>[2x]MFHSSAMVNSHRKPMFNIHRGFYCLTAILPQICICSQFSVPSSYHFTEDPGAFPVATNGERFPWQELRLPSVVIPLHYDLFVHPNLTSLDFVASEKIEVLVSNATQFIILHSKDLEITNATLQSEEDSRYMKPGKELKVLSYPAHEQIALLVPEKLTPHLKYYVAMDFQAKLGDGFEGFYKSTYRTLGGETRILAVTDFEPTQARMAFPCFDEPLFKANFSIKIRRESRHIALSNMPKVKTIELEGGLLEDHFETTVKMSTYLVAYIVCDFHSLSGFTSSGVKVSIYASPD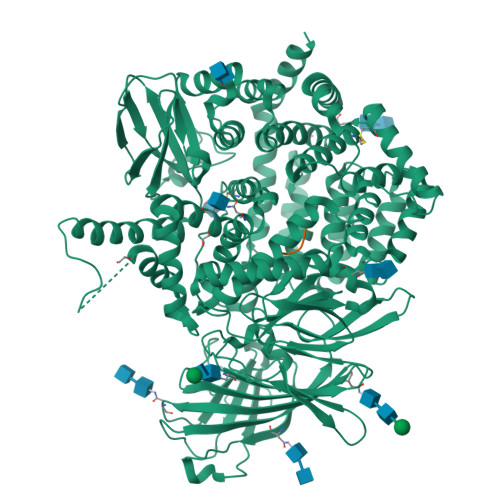KRNQTHYALQASLKLLDFYEKYFDIYYPLSKLDLIAIPDFAPGAMENWGLITYRETSLLFDPKTSSASDKLWVTRVIAHELAHQWFGNLVTMEWWNDIWLKEGFAKYMELIAVNATYPELQFDDYFLNVCFEVITKDSLNSSRPISKPAETPTQIQEMFDEVSYNKGACILNMLKDFLGEEKFQKGIIQYLKKFSYRNAKNDDLWSSLSNSCLESDFTSGGVCHSDPKMTSNMLAFLGENAEVKEMMTTWTLQKGIPLLVVKQDGCSLRLQQERFLQGVFQEDPEWRALQERYLWHIPLTYSTSSSNVIHRHILKSKTDTLDLPEKTSWVKFNVDSNGYYIVHYEGHGWDQLITQLNQNHTLLRPKDRVGLIHDVFQLVGAGRLTLDKALDMTYYLQHETSSPALLEGLSYLESFYHMMDRRNISDISENLKRYLLQYFKPVIDRQSWSDKGSVWDRMLRSALLKLACDLNHAPCIQKAAELFSQWMESSGKLNIPTDVLKIVYSVGAQTTAGWNYLLEQYELSMSSAEQNKILYALSTSKHQEKLLKLIELGMEGKVIKTQNLAALLHAIARRPKGQQLAWDFVRENWTHLLKKFDLGSYDIRMIISGTTAHFSSKDKLQEVKLFFESLEAQGSHLDIFQTVLETITKNIKWLEKNLPTLRTWLMVNTRHHHHHH;>GPGRAF[2x]> 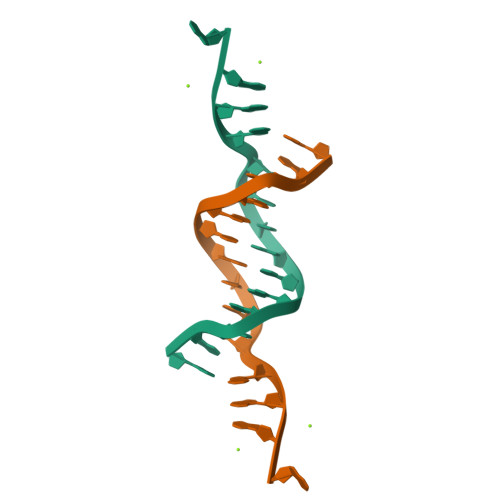GGAAATATTGGAGA> MSSAIKEVQGAPVKWVTNWTPEAIRGLVDQEKGLLDPRIYADQSLYELELERVFGRSWLLLGHESHVPETGDFLATYMGEDPVVMVRQKDKSIKVFLNQCRHRGMRICRSDAGNAKAFTCSYHGWAYDIAGKLVNVPFEKEAFCDKKEGDCGFDKAEWGPLQARVATYKGLVFANWDVQAPDLETYLGDARPYMDVMLDRTPAGTVAIGGMQKWVIPCNWKFAAEQFCSDMYHAGTTTHLSGILAGIPPEMDLSQAQIPTKGNQFRAAWGGHGSGWYVDEPGSLLAVMGPK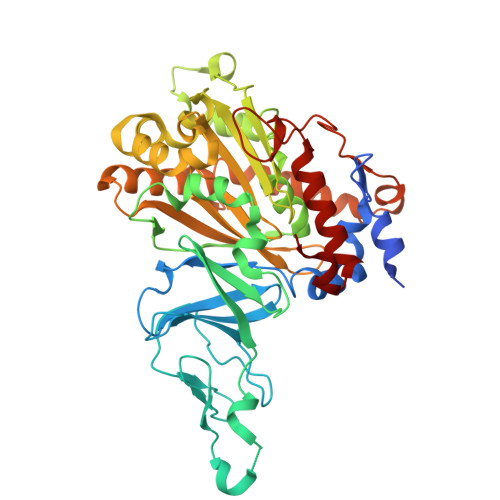VTQYWTEGPAAELAEQRLGHTGMPVRRMVGQHMTIFPTCSFLPAMNNIRIWHPRGPNEIEVWAFTLVDADAPAEIKEEYRRHNIRNFSAGGVFEQDDGENWVEIQKGLRGYKAKSQPLNAQMGLGRSQTGHPDFPGNVGYVYAEEAARGMYHHWMRMMSEPSWATLKP>MNHHYRDTRKIDPSRGATLGDGTPNDNDRIEIGPTQLAFSEWAAAGLQLPNLDRMREYRWKRLTQAIVDRGYGGLLMFDPLNIRYATDSTNMQLWNTHNPFRAVLLCADGYMVIWDYKNSPFLSKFNPLVREQRSGADLFYFDRGDKVDVQADVFANEVRVLMQDHAPGHTRLAVDKIMLHGLRALEAQGFEIMEGEEVTEKTRAIKGPDEILAMRCASHACETAVAEMEKFARAHVGDGKTSEDDIWAVLHAENIKRGGEWIETRLLASGPRTNPWFQECGPR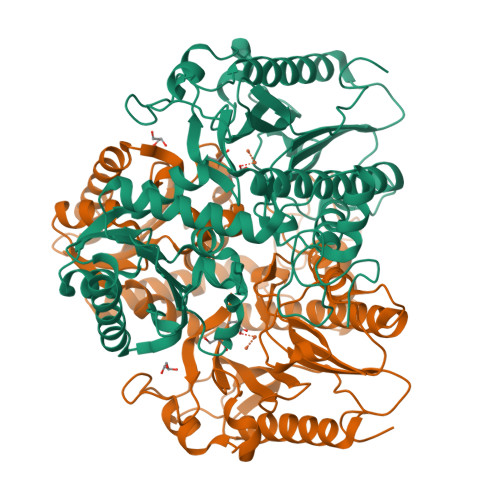ITQKNEIIAFDTDLIGSYGICVDISRTWWIGDQKPRPDMVYAMQHAHEHIMTNMEMLKPGVMIPDLTANCHRLDDKFQAQKAGCLMHGVGLCDEWPLVAYPDKAVPGSYDYPLEPGMVLCVEAAVGEVGGDFSIKLEDQVLITEDGYENLTTYPFDAALMGLA[4x]> 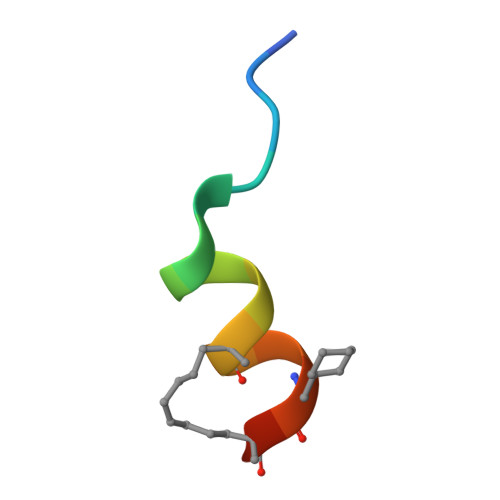LLPPTEQDLLKLALYX> SSPGKPPRLVGGPMDASVEEEGVRRALDFAVGEYNKASNDMYHSRALQVVRARKQIDAGVNYFLDVELGRTTCTKTQPNLDNCPFHDQPHLKRKAFCSFQIYAVPW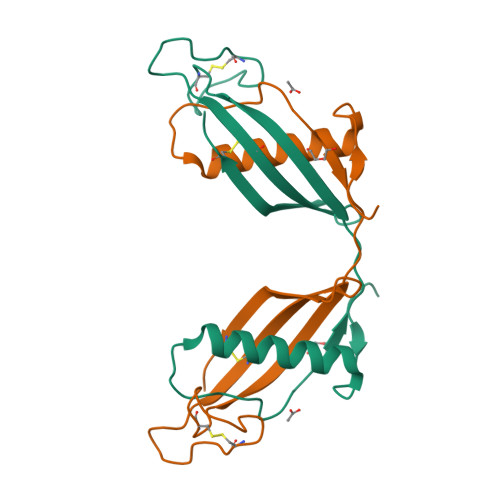QGTMTLSKSTCQDA> MSEDYYEKSTVSLTEKYKEFFKIGAAVTVKDFEGIHGRILTKHFNSLTPENDMKFERIHPKEDFYNFEATDKIKDFALKHNMQLRGHTLVWHNQTPEWVFRDNDKEAPKELVIERLREHIKTICTRYRDVVYSWDVVNAAVEDKTDVLLRDSKWRRIIGDDYIKIAFE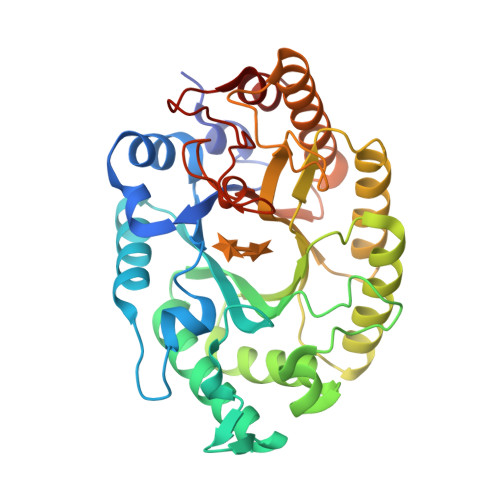IAKKYTGNGKLFYNDYNNEMPYKLEKTYKVLKSLLEEGTPIDGVGIQAHWNIWDKNLIDNLKRAIETYASLGLEIQITELDISVFEFEDRRTDLLEPTEEMVELQAKVYEDVFRVFREYRDVITSVTLWGISDRHTWKDNFPVIGRKDWPLLFDIDGKPKKAFFRIIDFL>[2x]MESCYNPGLDGIIEYDDFKLNSSIVEPKEPAPETADGPYLVIVEQPKQRGFRFRYGCEGPSHGGLPGASSEKGRKTYPTVKICNYEGPAKIEVDLVTHSDPPRAHAHSLVGKQCSELGICAVSVGPKDMTAQFNNLGVLHVTKKNMMGTMIQKLQRQRLRSRPQGLTEAEQRELEQEAKELKKVMDLSIVRLRFSAFLRASDGSFSLPLKPVISQPIHDSKSPGASN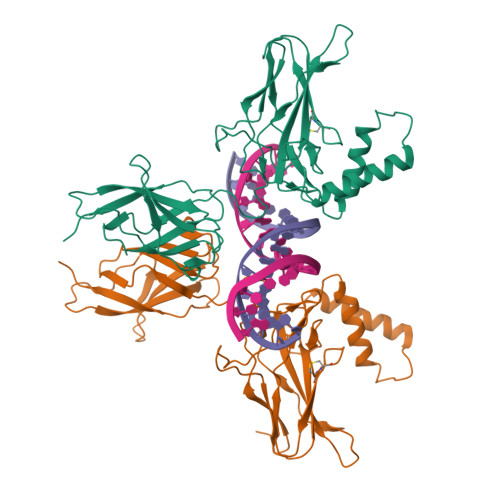LKISRMDKTAGSVRGGDEVYLLCDKVQKDDIEVRFYEDDENGWQAFGDFSPTDVHKQYAIVFRTPPYHKMKIERPVTVFLQLKRKRGGDVSDSKQFTYYPLVEDKEEVQRKRRKALPTFSQPFGGGSHMGGGSGGAAGGYGGAGGGGSLGFFPSSLAYSPYQSGAGPMGCY The recently identified bacterial Sir2 domain-containing protein, defense-associated sirtuin 2 (DSR2), recognizes the phage tail tube and depletes NAD+ to abort phage propagation, which is counteracted by the phage-encoded DSR anti-defense 1 (DSAD1), but their molecular mechanisms remain unclear. DSR2 contains an N-terminal Sir2 domain that serves as an NADase effector responsible for NAD+ hydrolysis, a C-terminal domain (CTD) that functions as a sensor for detecting invading phages (as discussed later), and a middle domain (MID) that connects the Sir2 effector and the CTD sensor. DSR2 forms a tetramer with its C-terminal sensor domains (CTDs) in two distinct conformations: CTDclosed or CTDopen. Monomeric, rather than oligomeric, tail tube proteins preferentially bind to CTDclosed and activate Sir2 for NAD+ hydrolysis.

To elucidate the structural basis for the NAD+ hydrolysis by the tube-activated DSR2, we incubated the substrate (1 mM NAD+) with DSR2H171A–tube complex, which was obtained by co-expression the catalytically inactive DSR2H171A mutant and tail tube proteins together in the same bacterial cells. We then determined the cryo-EM structure of the DSR2H171A–tube–NAD+ complex at 3.0-Å resolution, in which approximately 60% density was observed, facilitating the accurate tracing of the NAD+ substrates. Looking closely at the four densities corresponding to the NAD+ substrate, the densities representing the adenosine and adenosine-ribose moiety of NAD+ were well defined, while we observed a weak density corresponding to the nicotinamide and nicotinamide-ribose groups, suggesting the flexibility of the nicotinamide ribose of NAD+ when it binds to the DSR2–tube complex. However, we did not observe a clear density located in sites B and C; by contrast, bound NAD+ within the Sir2 domain of DSR2 adopts an orientation with a ~ 90° rotation compared to that seen with a nonhydrolyzable NAD+ analogue, carba-NAD+, which sits in a position ready for catalysis in yHst2 in yeast (Saccharomyces cerevisiae). Instead of being inserted into sites B and C, the nicotinamide-ribose and nicotinamide groups interacted with the small helical domain, with the nicotinamide moiety stacking with residue W60. In site A, we observed the stabilization of the adenine group through stacking interactions with residues Y282 and T52, while residue T248 forms a hydrogen-bonding interaction with the 2’-OH group of the adenine-ribose (left inset). Mutation of Y282 to alanine decreased DSR2 NADase activity by about 50%, whereas the T52A, T248A and W60A single mutants had a negligible effect on DSR2 NADase activity, highlighting the critical role of the Y282-mediated adenine stacking interaction in site A. Thus, we speculated that the observed NAD+ bound in the DSR2H171A–tube complex represents an inactive conformation.

>[4x]MVKVDLESKRYGEKLKEVFLMLDNNVVECIKEITESSRNGKLVFFVGAGVSTLSDYPQWWRLVDKYHEELYGSPKKGNYSSDEYLRIPQIFYNVKGEMAFDGILKDFFQVDKPTNPIHDKILAMNPAHVITTNYDNLIDTACWKRGKYFSVISAEEDVANATSSRYLLKVAGDFRKGFKGENVVLKEDDYLNYDQNYPLISNLMKTIIATHTIVFIGYGLGDYNINMLLNWVRKLQKDSFHKPFFIRTDPSPIENETLIYYENKGLRIIDAASLIDSNEYDYLERYSAVMDLLIESQENKFITKDDEVIDYIYGKISPLFALQYIRKIDLKHVFEYDYHFEVNGTVVRHKNKGFGYMERFFELKESCDERSKLSKKQYERFNALFNFFEKNGVICMAKDAGTLNTSIEINSLAYHGKYDVMKKFIEEQSVSIEDDYKKAFFLACLGRWEESYDLYSNIILNSIDESNGCVYYLSQINRYRIYQSITQAVTQFNGLGLLTFGRHYKPFTDEFLARIEREMTNFNIDDLFNGMPFEFQKKYKILEFLSDNQFLYDDTVKLFELTNKVRSEMSEGSYSFGMSSDIVVLLRLYDNLRFLYENCLWSVSFHEFHQYIRNSMSLLIEKAEYERTRDIDELGFSFFGKKSGFFMEYYDFVNISRHFKIDDIKNLERSCSIDKIRFGEQEKIEEYLVGIAEEITKQFSANGMNVVFYTQFISEAKAALYFAKYVKLSEEGLGKIVKALLFYFPERDLDIGKRYVWLERLTKCNELPKSIISIIDDFLVLQAEKHIDQNYSEVSSNGLYSRDYGALIKHFEKNFISKRLSEITLCLTQDKQKQIDFLFKLLPLLSTNAKSHLLSFKSVENINDLMNGIRIGLIDEFTPEHEELIIEYLETRKVNYIVEKEKGIQTFSSNDYMSTFGIWYFLEEINNSKMEEFIGMDDQYDFFVDPENFDYKKFIPSWLKNYNDKLLGKIAGNKHMKHHVIEVLKERVKNSNDKRYLEILMNYFI;>[2x]MKTVIQDTADVYFKRKSDGKLVFTAEAQTASFSQAISEEKLRGGIGNKPLYILKSEKEINLTVKNAFFDLEWLAMTQGETIQEETKVKVFDREHGLIVDDTNKVTLKGKPVSDVTFYNKKGLTYKIAVSTDGTYTIPTAFAAAKDKLTAVYQIEKVGRRLAIKASKFSERYEVEYRTIAYNPDTEEVYSDIYIQFPNVSPSGEFEMSLENGNALAPEIKFEALADTDTDEMAVVIEASRDENTAAPVEDTTGSTQSSDLGGTTE>MSKNYHIAVLPGDGIGPEVMTQALKVLDAVRNRFAMRITTSHYDVGGAAIDNHGQPLPPATVEGCEQADAVLFGSVGGPKWEHLPPDQQPERGALLPLRKHFKLFSNLRPAKLYQGLEAFCPLRADIAANGFDILCVRELTGGIYFGQPKGREGSGQYEKAFDTEVYHRFEIERIARIAFESARKRRHKVTSIDKANVLQSSILWREIVNEIATEYPDVELAHMYIDNATMQLIKDPSQFDVLLCSNLFGDILSDECAMITGSMGMLPSASLNEQGFGLYEPAGGSA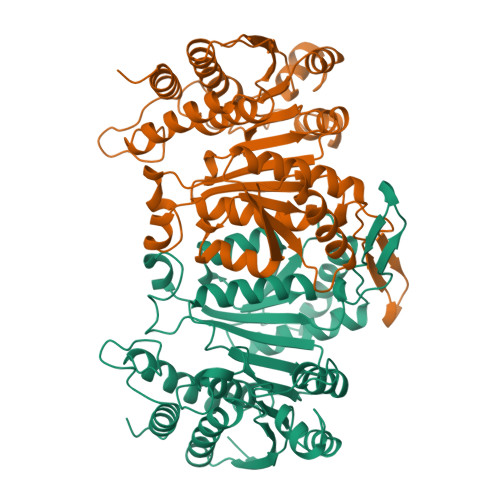PDIAGKNIANPIAQILSLALLLRYSLDADDAACAIERAINRALEEGIRTGDLARGAAAVSTDEMGDIIARYVAEGV[2x]> MAVISKVTYSLYDQKEINATDIIISHVKNDDDIGTVKDGRLGAMDGALCKTCGKTELECFGHWGKVSIYKTHIVKPEFISEIIRLLNHICIHCGLLRSREPYSDDINLKELSGHALRRLKDKILSKKKSCWNSECMQPYQKITFSKKKVCFVNKLDDINVPNSLIYQKLISIHEKFWPLLEIHQYPANLFYTDYFPIPPLIIRPAISFWIDSIPKETNELTYLLGMIVKNCNLNADEQVIQKAVIEYDDIKIISNNTTSINLSYITSGKNNMIRSYIVARRKDQTARSVIGPSTSITVNEVGMPAYIRNTLTEKIFVNAFTVDKVKQLLASNQVKFYFNKRLNQLTRIRQGKFIKNKIHLLPGDWVEVAVQEYTSIIFGRQPSLHRYNVIASSIRATEGDTIKISPGIANSQNADFDGDEEWMILEQNPKAVIEQSILMYPTTLLKHDIHGAPVYGSIQDEIVAAYSLFRIQDLCLDEVLNILGKYGREFDPKGKCKFSGKDIYTYLIGEKINYPGLLKDGEIIANDVDSNFVVAMRHLSLAGLLSDHKSNVEGINFIIKSSYVFKRYLSIYGFGVTFKDLRPNSTFTNKLEAINVEKIELIKEAYAKYLNDVRDGKIVPLSKALEADYVESMLSNLTNLNIREIEEHMRQTLIDDPDNNLLKMAKAGYKVNPTELMYILGTYGQQRIDGEPAETRVLGRVLPYYLPDSKDPEGRGYILNSLTKGLTGSQYYFSMLVARSQSTDIVCETSRTGTLARKIIKKMEDMVVDGYGQVVIGNTLIKYAANYTKILGSVCKPVDLIYPDESMTWYLEISALWNKIKQGFVYSQKQKLAKKTLAPFNFLVFVKPTTEDNAIKVKDLYDMIHNVIDDVREKYFFTVSNIDFMEYIFLTHLNPSRIRITKETAITIFEKFYEKLNYTLGGGTPIGIISAQVLSEKFTQQALSSFHTTEKSGAVKQKLGFNEFNNLTNLSKNKTEIITLVSDDISKLQSVKINFEFVCLGELNPNITLRKETDKYVVDIIVNRLYIKRAEITELVVEYMIERFISFSVIVKEWGMETFIEDEDNIRFTVYLNFVEPEELNLSKFMMVLPGAANKGKISKFKIPISDYTGYDDFNQTKKLNKMTVELMNLKELGSFDLENVNVYPGVWNTYDIFGIEAAREYLCEAMLNTYGEGFDYLYQPCDLLASLLCASYEPESVNKFKFGAASTLKRATFGDNKALLNAALHKKSEPINDNSSCHFFSKVPNIGTGYYKYFIDLGLLMRMERKLSDKISSQKIKEMEETEDF;> MKKNTNSEMDQRLGYKFLVPDPKAGVFYRPLHFQYVSYSNFILHRLHEILTVKRPLLSFKNNTERIMIEISNVKVTPPDYSPIIASIKGKSYDALATFTVNIFKEVMTKEGISITKISSYEGKDSHLIKIPLLIGYGNKNPLDTAKYLVPNVIGGVFINKQSVEKVGINLVEKITTWPKFRVVKPNSFTFSFSSVSPPNVLPTRYRHYKISLDISQLEALNISSTKTFITVNIVLLSQYLSRVSLEFIRRSLSYDMPPEVVYLVNAIIDSAKRITESITDFNIDTYINDLVEAEHIKQKSQLTINEFKYEMLHNFLPHMNYTPDQLKGFYMISLLRKFLYCIFHTSRYPDRDSMVCHRILTYGKYFETLAHDELENYIGNIRNDIMNNHKNRGTYAVNIHVLTTPGLNHAFSSLLSGKFKKSDGSYRTHPHYSWMQNISIPRSVGFYPDQVKISKMFSVRKYHPSQYLYFCSSDVPERGPQVGLVSQLSVLSSITNILTSEYLDLEKKICEYIRSYYKDDISYFETGFPITIENALVASLNPNMICDFVTDFRRRKRMGFFGNLEVGITLVRDHMNEIRINIGAGRLVRPFLVVDNGELMMDVCPELESRLDDMTFSDIQKEFPHVIEMVDIEQFTFSNVCESVQKFRMMSKDERKQYDLCDFPAEFRDGYVASSLVGINHNSGPRAILGCAQAKQAISCLSSDIRNKIDNGIHLMYPERPIVISKALETSKIAANCFGQHVTIALMSYKGINQEDGIIIKKQFIQRGGLDIVTAKKHQVEIPLENFNNKERDRSNAYSKLESNGLVRLNAFLESGDAMARNISSRTLEDDFARDNQISFDVSEKYTDMYKSRVERVQVELTDKVKVRVLTMKERRPILGDKFTTRTSQKGTVAYVADETELPYDENGITPDVIINSTSIFSRKTISMLIEVILTAAYSAKPYNNKGENRPVCFPSSNETSIDTYMQFAKQCYEHSNPKLSDEELSDKIFCEKILYDPETDKPYASKVFFGPIYYLRLRHLTQDKATVRCRGKKTKLIRQANEGRKRGGGIKFGEMERDCLIAHGAANTITEVLKDSEEDYQDVYVCENCGDIAAQIKGINTCLRCSKLNLSPLLTKIDTTHVSKVFLTQMNARGVKVKLDFERRPPSFYKPLDKVDLKPSFLV;> MQHPREENSIVVELEPSLATFIKQGFNNLVKWPLLNIGIVLSNTSTAVNEEWLTAVEHIPTMKIFYKHIHKILTREMGFLVYLKRSQSERDNYITLYDFDYYIIDKDTNSVTMVDKPTELKETLLHVFQEYRLKSSQTIELIAFSSGTVINEDIVSKLTFLDVEVFNREYNNVKTIIDPDFVFRSPFIVISPMGKLTFFVEVYSWFDFKSCFKDIIDFLEGALIANIHNHMIKVGNCDETVSSYNPESGMLFVNDLMTMNIVNFFGCNSRLESYHRFDMTKVDVELFIKALSDACKKILSASNRL;> MNQYNVKYLAKILCLKTEIARDPYAVINRNVLLRYTTDIEYNDLVTLITVRHKIDSMKTVFQVFNESSINYTPVDDDYGEPIIITSYLQKGHNKFPVNFLYIDVVISDLFPSFVRLDTTETNIVNSVLQTGDGKKTLRLPKMLETEIVVKILYRPNIPLKIVRFFRNNMVTGVEIADRSVISVAD;> MADTDDIIDYESDDLTEYEDDEEEEEDGESLETSDIDPKSSYKIVESASTHIEDAHSNLKHIGNHISALKRRYTRRISLFEIAGIIAESYNLLQRGRLPLVSEFSDETMKQNMLHVIIQEIEEGSCPIVIEKNGELLSVNDFDKDGLKFHLDYIIKIWKLQKRY;> MSSFVTNGYLSVTLEPHELTLDIKTNIRNAVYKTYLHREISGKMAKKIEIREDVELPLGEIVNNSVVINVPCVITYAYYHVGDIVRGTLNIEDESNVTIQCGDLICKLSRDSGTVSFSDSKYCFFRNGNAYDNGSEVTAVLMEAQQGIESSFVFLANIVDS;>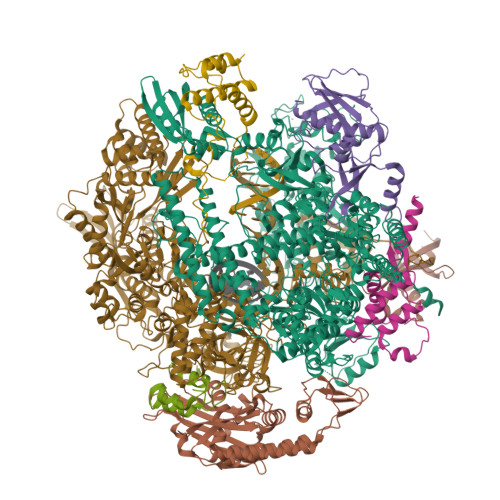 MVFQLVCSTCGKDISHERYKLIIRKKSLKDVLVSVKNECCRLKLSTQIEPQRNLTVQPLLDIN;> MENVYISSYSSNEQTSMAVAATDIRELLSQYVDDANLEDLIEWAMEKSSKYYIKNIGNTKSNIEETKFESKNNIGIEYSKDSRNKLSYRNKPSIATNLEYKTLCDMIKGTSGTEKEFLRYLLFGIKCIKKGVEYNIDKIKDVSYNDYFNVLDEKYNTPCPNCKSRNTTPMMIQTRAADEPPLVRHACRDCKQHFKPPKFRAFRNLNVTTQSIHENKEITEILPDNNPSPPESPEPASPIDDGLIRATFDRNDEPPEDDE>[4x]MRNGLLKVAALAAASAVNGENLAYSPPFYPSPWANGQGDWAEAYQKAVQFVSQLTLAEKVNLTTGTGWEQDRCVGQVGSIPRLGFPGLCMQDSPLGVRDTDYNSAFPAGVNVAATWDRNLAYRRGVAMGEEHRGKGVDVQLGPVAGPLGRSPDAGRNWEGFAPDPVLTGNMMASTIQGIQDAGVIACAKHFILYEQEHFRQGAQDGYDISDSISANADDKTMHELYLWPFADAVRAGVGSVMCSYNQVNNSYACSNSYTMNKLLKSELGFQGFVMTDWGGHHSGVGSALAGLDMSMPGDIAFDSGTSFWGTNLTVAVLNGSIPEWRVDDMAVRIMSAYYKVGRDRYSVPINFDSWTLDTYGPEHYAVGQGQTKINEHVDVRGNHAEIIHEIGAASAVLLKNKGGLPLTGTERFVGVFGKDAGSNPWGVNGCSDRGCDNGTLAMGWGSGTANFPYLVTPEQAIQREVLSRNGTFTGITDNGALAEMAAAASQADTCLVFANADSGEGYITVDGNEGDRKNLTLWQGADQVIHNVSANCNNTVVVLHTVGPVLIDDWYDHPNVTAILWAGLPGQESGNSLVDVLYGRVNPGKTPFTWGRARDDYGAPLIVKPNNGKGAPQQDFTEGIFIDYRRFDKYNITPIYEFGFGLSYTTFEFSQLNVQPINAPPYTPASGFTKAAQSFGQPSNASDNLYPSDIERVPLYIYPWLNSTDLKASANDPDYGLPTEKYVPPNATNGDPQPIDPAGGAPGGNPSLYEPVARVTTIITNTGKVTGDEVPQLYVSLGGPDDAPKVLRGFDRITLAPGQQYLWTTTLTRRDISNWDPVTQNWVVTNYTKTIYVGNSSRNLPLQAPLKPYPGI

The GH3 Cel3A from the thermophilic fungus Rasamsonia emersonii (ReCel3A) is a more efficient additive to enzyme mixtures compared with HjCel3A. Biochemical characterization of ReCel3A revealed a substrate preference for disaccharides over longer oligosaccharides. The GH family 3 BGL Cel3A from R. emersonii is an efficient supplement to whole cellulase mixtures for the production of fermentable sugars from lignocellulosic biomass. We also present the three-dimensional crystal structure of Cel3A from the moderately thermophilic filamentous fungus R. emersonii solved to 2.2 Å resolution.

The crystal structure of ReCel3A is a tetramer composed of two biological dimers. The large number of hydrogen bonds between the protein and the ligand bound in the catalytic centre makes the binding in subsite −1 of GH3 enzymes highly specific. The two catalytic residues in ReCel3A were identified based on homology to other GH3 structures: Asp277 (nucleophile) and Glu505 (acid/base). In the ReCel3A structure, clear density is observed for a glucose unit in the −1 subsite and no indication of distortion from the relaxed chair conformation can be observed. When compared with the corresponding residues in HjCel3A, the plane of the Trp68 side chain has turned almost 90° away from the +1 subsite. This allows aromatic stacking of the Phe302 and Trp68 side chains to form a hydrophobic ‘knob’ and places the phenylalanine residue in the +1 subsite rather than in the +2 subsite as in HjCel3A. The lack of a +2 subsite in ReCel3A could explain the activity profile for the enzyme as a more pronounced cellobiase than HjCel3A. The dimer interface has a total overall contact area of 1572 Å2, to which the modelled N-glycans contribute about 19%. The N-glycosylation chain IV shows the remarkable feature of being buried by the extended C-terminal loop. Two conserved aromatic residues, Tyr720 and Tyr727, on the loop provide stacking interactions with the two buried NAG residues 1201 and 1202.>GPGADRAQDHNNNNTPRNSNYVVEEEEVSEEEEEAIMMPDFGDHVDTSIFGQILEMDEGDDHDFSAPLVLNFFEQAEETFQKMETALNNKDLPELSKLGHFLKGSSATLGFTKIRDSCQLIQQYGHGLNVDGSSEPDEGVCLKKIAEALASARVDTVALHKMMREFFEY[4x]

If the HK incorporates a REC domain (REC-1) is denoted as hybrid histidine kinase (hHK), and the first His-Asp phosphotransfer event occurs in the same polypeptide chain. Then, HPt protein containing a phosphorylatable His shuffles the phosphoryl group from the phosphorylatable Asp in the REC-1 domain to the phosphorylatable Asp in the REC domain of an RR (REC-2) in two more phosphotransfer steps. In fungi, the HPt accepts the phosphoryl group from REC-1 domains of various hHKs upstream of the signaling pathway and forwards it downstream to REC-2 domains present in at least two conserved RRs, Ssk1 and Skn7. Also, we have obtained the crystal structures of Ct_HPt alone and in complex with REChHK6 bound to the phosphomimetic BeF3−, as well as the crystal structures of REChHK3 and RECCa_Sln1.

To analyze differences in the structure of Ct_HPt before and after binding to REChHK6, we obtained the crystal structure of isolated Ct_HPt. It contained four molecules in the AU and each molecule contributed to an interface area of ~800 Å2 between two molecules. The interface area contained several salt bridges between two Arg residues located in αE (R158 and R169) and two Glu residues located in αB (E82 and E89). Interestingly, R158 formed intrachain salt bridges with E82 and E89, as well as an interchain salt bridge with E82, while R169 formed an interchain salt bridge with E89. According to the EPPIC and PISA servers this interface was the result of crystal packing and SEC-MALS analysis with Ct_HPt indicated a MW of 18.1 kDa (theoretical MW is 18.7 kDa) demonstrating the presence of the monomeric species in solution. Finally, the structural comparison between Ct_HPt isolated and bound to REChHK6 demonstrated high structural similarity between them (rmsd of ~0.9 Å for 129 residues), although slight structural changes were observed in the N-terminal region, αA, loop αA–αB and loop αD–αE. Meanwhile, the intrachain salt bridge nucleated by R158 in αE with E82 and E89 in αB is also present and has not been disturbed. This fact indicates that Ct_HPt shows little plasticity, a useful conserved feature to be recognized similarly by several REC-1 domains. Finally, our studies have uncovered two salt bridges in Ct_HPt between two Glu residues in αB and an Arg residue in αE that provide bundle stability. As these residues seem rather conserved between human fungal pathogens, except in S. cerevisiae, we envision that these salt bridges could be present in other HPt proteins. These salt bridges do not intervene in complex recognition but seem to provide bundle stability preventing conformational plasticity.>[2x]MKKRVVKLRELVPAVAALAVAVLIQSATGSSGGSGHTPTTQATHADDHDLTTHNGTEEHDDGHDDGHDDLHAHAPKVIVFISGSCLFGAISRSLFKKLPIPYTVVLLILGAILGVVASNVPLVEEHTRDVAHMDPHVLLQIFLPVLIFESAFAMDVHTFMRSFSQVCILALFGLVVASVLTAVLAMNLFNYNWNFSEAMMFGAIMSATDPVAVVALLKDLGASKQLGTIIEGESLLNDGCAIVIFNVFMKMVFFPQLTSTVGQNVLYFLQVAVAGPLWGYAVAKVTVFFLSHIFNDALVEITITLAATYLTYYIGDIWLEVSGVLAVVVLGLIVNAEKTSISPEVEVFLHRFWEMLAYLANTLIFMMVGVVVTQKALVAVDKMDWFYLIILYLAITIIRGMVISLFSPILSRIGYGLTWRNAVIMTWGGLRGAVGLALALVVENLAGNDVIGSKFLFHTAGIVVLTLVINATTIQTLLRILGMSDISIPKRLAMAGAVRRIHEGQNRTLNMLKSDRFLADADWDIATAACEISDPYSALSDDENAPADELTLGERKSVCPGCKAMVPNEPSPREFADMMEEARLRMLKAEKISYWKQFEHGMLAREALRLLVQHAEVAADEKDQFILVDDLKKSWQIKGIYPWLKRKLEDLISEKKIAAIPMPKYKLGKLMYKICHHMAFEVTINIAIVLNIVPIIMEFVVQDKMASVSTMAAPGSTVSSEPSSLQKIEDALRISNYVFFVIYAIEAIVKILGLGRHYIVSHWNKFDAFILVVALVDIIIAETLLKGSITINLSSIKVVKLFRLLRGLRMLRLTKALIPKLILVVNGKINNQLSLGYDVGKGYIIGEEEVGKIIDRMVDNKKILRELKHISETGRLQVVKELGLLQREHPGIAVSVKTRQAIRTILNHSRETIHELQGAGLLDEMEAHKLELTVEIKMKRLMNAPSSIPPPPPENLLKNVSWLAGDMKLIDFIKARASLLHFDYGEVIVREGDESDGLFLIVSGLVKLYGKSAFLDHDNPPVTAGSEENEVFEDYLTVGNVIGEMGVLTKKPRNATVTCETTVQVYFITAEDMNIAIDTFTLYPSLEYRLWRVVAIRIATPLIMEQMAFQGWTQEKVKLHLERGYLVDLAESHFQFNIDATLEDVILINGTAYNAHTREEIRSPCLISRTVHKLTFQYTATEEPRLFVVRNAEYNGPILDGRLDVDSKRSLISITEISSNMCLKHAAELRQKNSKVMLSRKSSGAAAKEEEDCIPNTSDVEQAAGVSPSVPTKTTPKPKSFLPSLGLSMSKERVNGEAVEESPVKTKQGEETPETEEGAAPRVNVENLYFQ

SLC9C1 belongs to the NHE family of ion transporters, which facilitate the electroneutral exchange of cations (Na+/Li+/K+) and protons (H+) across membranes to regulate intracellular pH, sodium levels and cell volume. Rather than containing a partially disordered cytoplasmic tail, it contains four additional TM helices that form an S1–S4 voltage-sensing domain (VSD), and a distal cyclic-nucleotide-binding domain (CNBD)2,4. The S4 VSD renders SLC9C1 a transporter that is activated only in response to hyperpolarization (−95 mV), and the CNBD bind cAMP to enable SLC9C1 to become activated closer to the resting membrane potential of sperm (−50 mV)2 VSDs are thought to have evolved independently from ion channels, and there are a few examples of non-channel VSD domains coupled to soluble enzymes. SLC9C1 is therefore an essential component of the pH–sAC–cAMP signalling pathway in metazoa, required for sperm motility and fertilization.

To understand the molecular basis of cAMP regulation, we determined the cryo-EM structure of SLC9C1 in the presence of cAMP, which was built into the EM maps reconstructed to 3.6 Å. Consistent with SLC9C1 being inactive at 0 mV, we observed no structural differences in the NHE transporter module. The CNBDs could not be modelled, with either absent or poor map features for the CNBDs at lower contour levels, and this decreased the size of the modelled cytoplasmic interface. Consistent with this interpretation, S4 and the connecting ICH3, ICH4 and ICH5 helices have moved outwards from their previously modelled position. The movement of the ICH3–ICH6 helices in the presence of cAMP is propagated to the VSD domains and increases their mobility. As such, cryo-EM map density for only one of the VSD domains was observed and at a lower local resolution of about 3.5 to 6.5 Å resolution. Comparing the VSD domain in the presence and absence of cAMP showed that there is an anti-clockwise displacement of S1–S3 helices on the intracellular side of around 7.5 to 10 Å. The detachment of ICH7 from the transporter module is clearly correlated with the repositioning of S4 and the VSD. Thus, it appears that cAMP has primed SLC9C1 for activation by detaching CNBD interactions with the cytoplasmic end of S4. However, the binding of cAMP to the CNBDs, appears to make it easier for the S4 helix to move downwards by (1) destabilizing S4–CNBD interactions; (2) weakening homodimerization contacts; and (3) partially detaching ICH7 and rearranging S1–S3 to facilitate S4 movement.> GSNIEQYIHDLDSNSFELDLQFSEDEKRLLLEKQAGGNPWHQFVENNLILKMGPVDERKGLFARRRQLLLTEGPHLYYVDPVNKVLKGEIPWSQELRPEAKNFKTFFVHTPNRTYYLMDP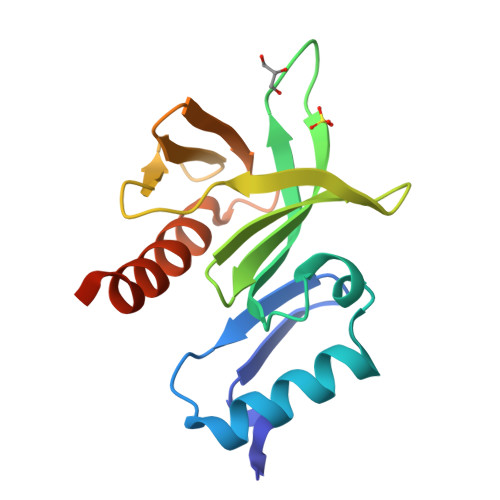SGNAHKWCRKIQEVWRQRYQSHPDAAVQ>GCGUC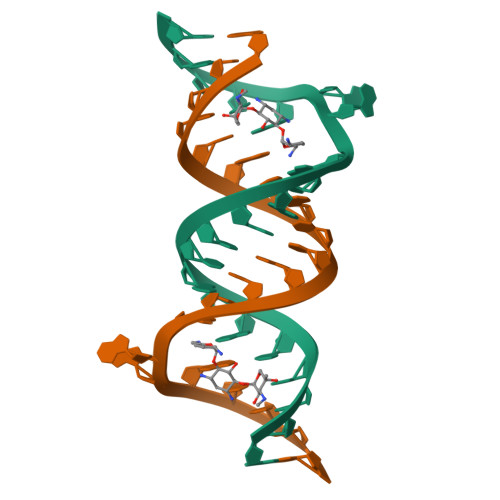ACACCGGUGAAGUCGC[2x]> TEFLKPRLVDIEQVSSTHAKVTLEPLERGFGHTLGNALRRILLSSMPGCAVTEVEIDGVLHEYSTKEGVQEDILEILLNLKGLAVRVQGKDEVILTLNKSGIGPVTAADITHDGDVEIVKPQH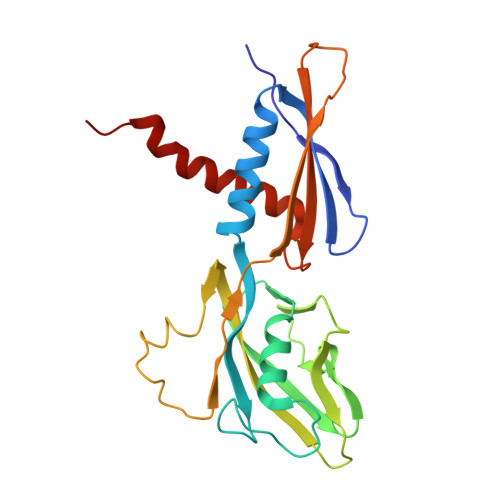VICHLTDENASISMRIKVQRGRGYVPASTRIHSEEDERPIGRLLVDACYSPVERIAYNVEAARVEQRTDLDKLVIEMETNGTIDPEEAIRRAATILAEQLEAFVDLRD> MIFFYATLLIGIAGIITFIRLALGPTVPDRVVAVDTLNTLIVAIMLLLGAAYERAIYIDIAIVYALLSYVGTLVIAKYLQG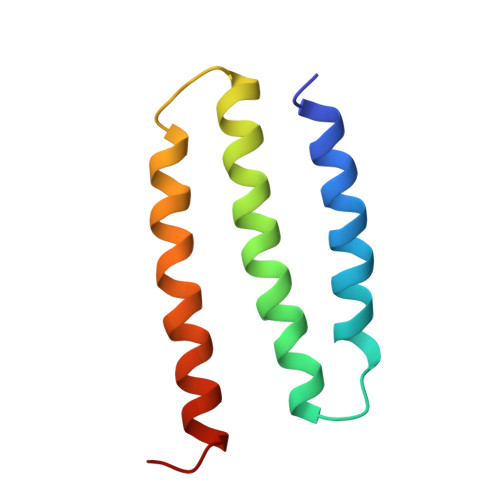GLQ> SEACVSVTSSILSSMDPTVDPCHDFFSYACGGWIKANPVPDGHSRWGTFSNLWEHNQAIIKHLLENSTASVSEAERKAQVYYRACMNETRIEELRAKPLMELIERLGGWNITGPWAKDNFQDTLQVVTAHYRTSPFFSVYVSADSKNSNSNVIQVDQSGLGLPSRDYYLNKTENEKVLTGYLNYMVQLGKLLGGGDEEAIRPQMQQILDFETALANITIPQEKRRDEELIYHKVTAAELQTLAPAINWLPFLNTIFYPVEINESEPIVVYDKEYLEQISTLINTTDRCLLNNYMIWNLVRKTSSFLDQRFQDADEKFMEVMYGTKKTSLPRWKFCVSDTENNLGFALGPMFVKATFAEDSKSIATEIILEIKKAFEESLSTLKWMDEETRKSAKEKADAIYNMIGYPNFIMDPKELDKVFNDYTAVPDLYFENAMRFFNFSWRVTADQLRKAPNRDQWSMTPPMVNAYYSPTKNEIVFPAGILQAPFYTRSSPKALNFGGIGVVVGHELTHAFDDQGREYDKDGNLRPWWKNSSVEAFKRQTECMVEQYSNYSVNGEPVNGRHTLGENIADNGGLKAAYRAYQNWVKKNGAEHSLPTLGLTNNQLFFLGFAQVWCSVRTPESSHEGLIT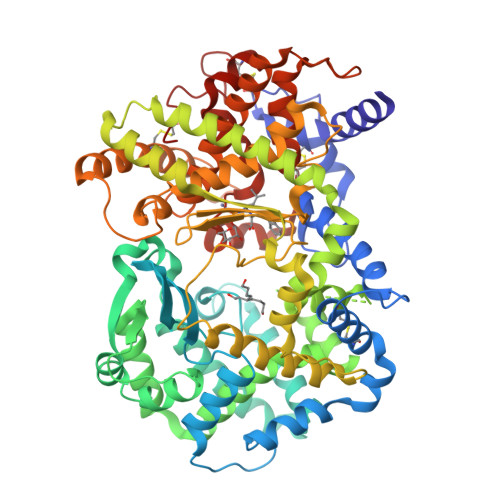DPHSPSRFRVIGSLSNSKEFSEHFRCPPGSPMNPPHKCEVW Sialylated precision glycomacromolecule | C92 H141 N21 O37 | 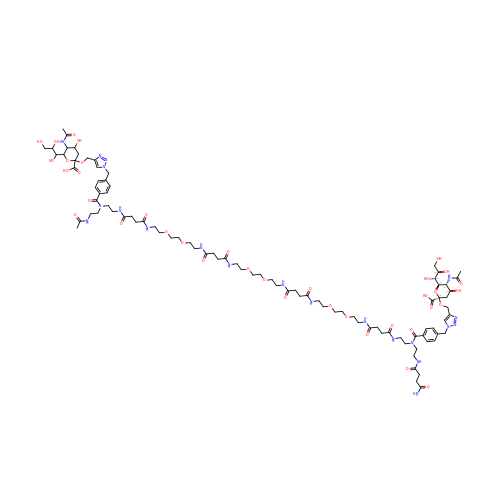DQKPDFSADBRBDM-WDGKASGMSA-N> MTAPHDVPDLTGSGEYLVPDVLQPGLTLVLVGTAPSGISARARAYYANPENKFWRTLHAVGLTPRQLVPQEYATLPQYGLGLTDVAKRHSGVAAALPGEAWRPDELRRKVEHYRPRIVAFTSKRGASETLG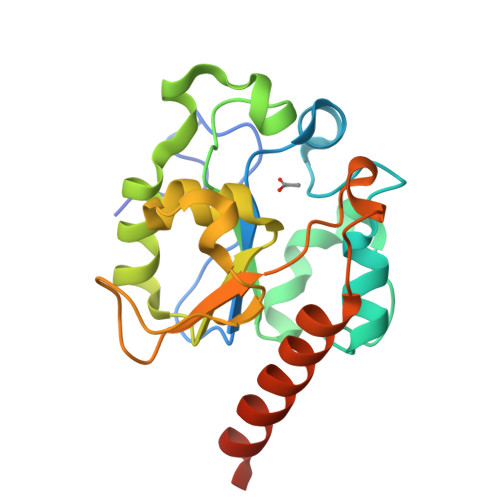VPTGKLPYGPQPQPLDWPAETELWVLPSTSPLGHNHFRLEPWQALGDRVRELRGAAEAGNPSPETPVL> MSVVSQVILQADDQLRYPTSGELKGIQAFLTTGAQRIRIAETLAENEKK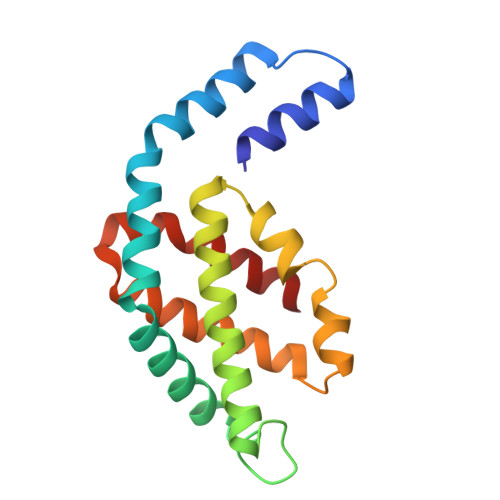IVDQAQKQLFKKHPEYRAPGGNAYGQRQYNQCLRDYGWYLRLVTYGVLAGNKEPIETTGLIGVKEMYNSLNVPVPGMVDAVTVLKDAALGLLSAEDANETAPYFDYIIQFMS> MLEKVETFDMNRVIDEFDEMTRNAHQVQKQTLKEILLKNQSAIYLQNCGLNGNATDPEEAFKSMVPLVTDVELEPYIKRMVDGDTSPILTGHPVPAISLSSGTSQGRPKFIPFTDELMENTLQLFRTAFAFRNRDFPIDDNGKALQFIFSSKQYISTGGVPVGTATTNVYRNPNFKAGMKSITSPSCSPDEVIFSPDVHQALYCHLLSGILFRDQVQYVFAVFAHGLVHAFRTFEQVWEEIVTDIKDGVLSNRITVPSVRTAMSKLLTPNPELAETIRTKCMSLSNWYGLIPALFPNAKYVYGIMTGSMEPYVPKLRHYAGDLPLVSHDYGSSEGWIAANVTPRLSPEEATFAVIPNLGYFEFLPVSETGEGEEKPVGLTQVKIGEEYEVVITNYAGLYRYRLGDVVKVIGFYNNTPQLKFICRRNLILSINIDKNTERDLQLSVESAAKRLSEEKIEVIDFSSYIDVSTDPGHYAIFWEISGETNED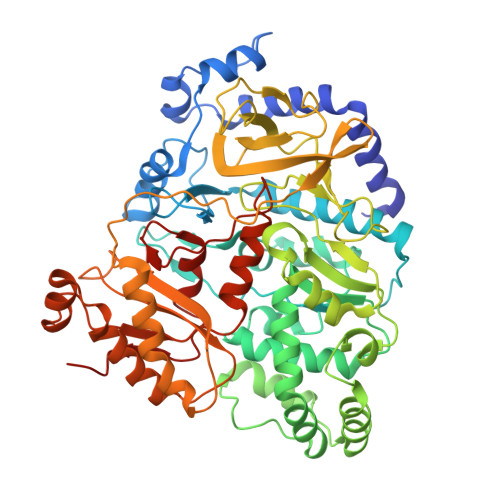VLQDCCNCLDRAFIDAGYVSSRKCKTIGALELRVVAKGTFRKIQEHFLGLGSSAGQFKMPRCVKPSNAKVLQILCENVVSSYFSTAF>MHHHHHHSLTDLVEQPAKVMRIGTMIKQLLEEVRAAPLDEASRNRLR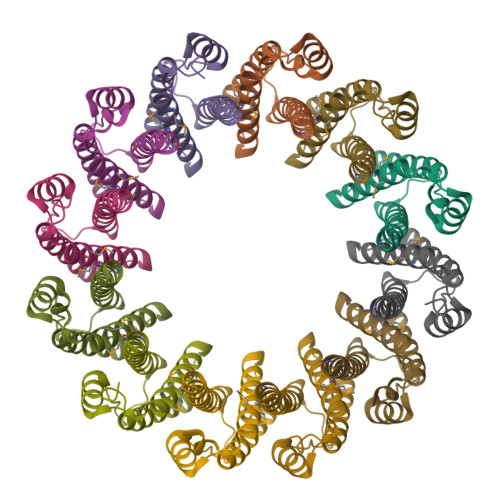DIHATSIRELEDGLAPELREELDRLTLPFNEDAVPSDAELRIAQAQLVGWLEGLFHGIQTALFAQQMAARAQLQQMRQGALPPG[4x]> VSVSEIRKAQRAEGPATILAIGTANPANCVEQSTYPDFYFKITNSEHKTELKEKFQRMCDKSMIKRRYMYLTEEILKENPNVCEYMAPSLDARQDMVVVEVPRLGKEAAVKAIKEWGQPKSKITHLIVCTTSGVDMPGADYQLTKLLGLRPYVKRYMMYQQGCFAGGTVLRLAKDLAENNKGARVLVVCSEVTAVTFRGPSDTHLDSLVGQALFGDGAAALIVGSDPVPEIEKPIFEMVWTAQTIAPDSEGAIDGHLREAGLTFHLLKDVPGIVSKNITKALVEAFEPLGISDYNSIFWIAHPGGPAILDQVEQKLALKP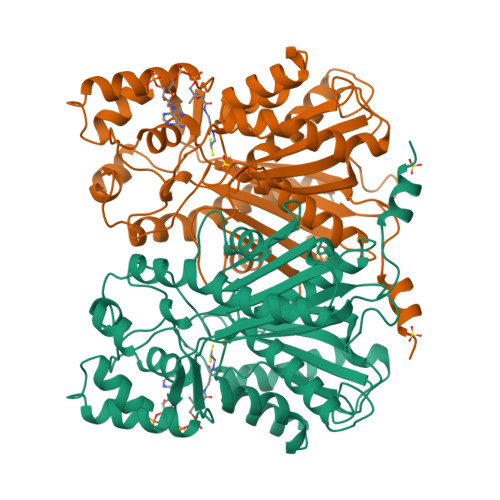EKMNATREVLSEYGNMSSACVLFILDEMRKKSTQNGLKTTGEGLEWGVLFGFGPGLTIETVVLRSVAI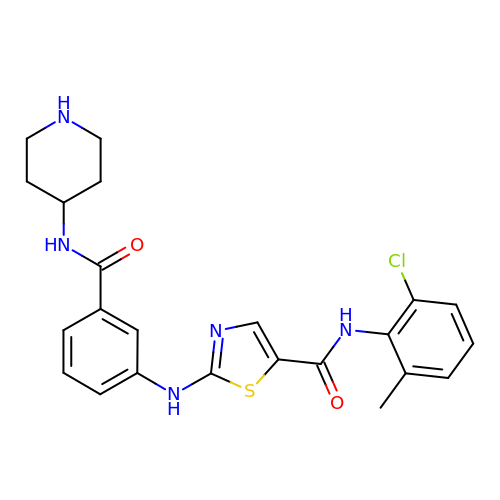~{N}-(2-chloranyl-6-methyl-phenyl)-2-[[3-(piperidin-4-ylcarbamoyl)phenyl]amino]-1,3-thiazole-5-carboxamide | C23 H24 Cl N5 O2 S | CCCAUTZOBQTZLJ-UHFFFAOYSA-N>[4x]MGATTTTHELNVSNSMTVGQYSSDFTLNGFTFITGGSIWEVDSSSRSYGGVNFTQRVKSGGK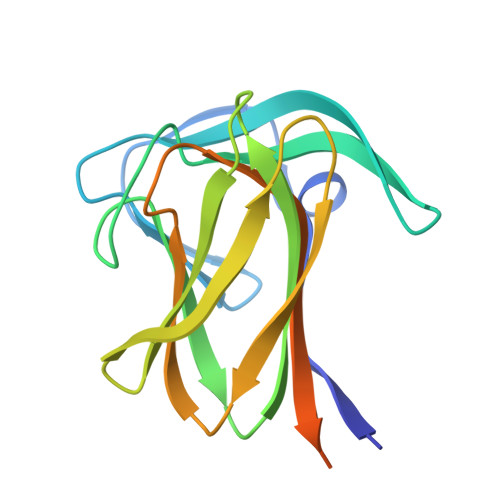GTISKRAISFTASGAGQLTVYAMSSGSTSRNVTLYGNGKDLESFTAVQDVITAMNFTIPNSGTYVIYPPDDGISYYYLKVVKTDSTPTPTPTVKPTQTPTPTPTLEHHHHHH>MSRLERLTSLNVVAGSDLRRTSIIGTIGPKTNNPETLVALRKAGLNIVRMNFSHGSYEYHKSVIDNARKSEELYPGRPLAIALDTKGPEIRTGTTTNDVDYPIPPNHEMIFTTDDKYAKACDDKIMYVDYKNITKVISAGRIIYVDDGVLSFQVLEVVDDKTLKVKALNAGKICSHKGVNLPGTDVDLPALSEKDKEDLRFGVKNGVHMVFASFIRTANDVLTIREVLGEQGKDVKIIVKIENQQGVNNFDEILKVTDGVMVARGDLGIEIPAPEVLAVQKKLIAKSNLAGKPVICATQMLESMTYNPRPTRAEVSDVGNAILDGADCVMLSGETAKGNYPINAVTTMAETAVIAE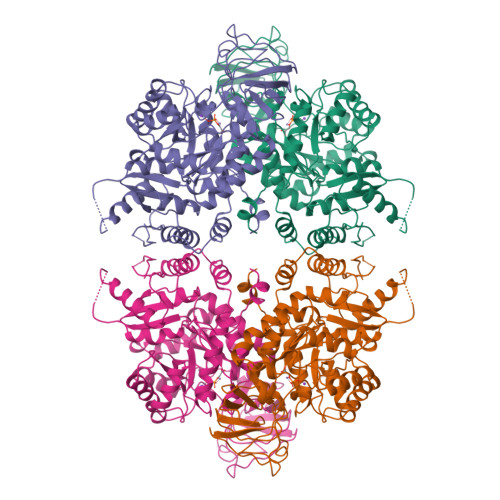QAIAYLPNYDDMRNCTPKPTSTTETVAASAVAAVFEQKAKAIIVLSTSGTTPRLVSKYRPNCPIILVTRCPRAARFSHLYRGVFPFVFEKEPVSDWTDDVEARINFGIEKAKEFGILKKGDTYVSIQGFKAGAGHSNTLQVSTV[2x]> MLQFEIDDEMEPLYNQAKQMRYGDYMKSTFKEDHSLEHRCVESAKIRAKYPDRVPVIVEKVSGSQIVDIDKRKYLVPSDITVAQFMWIIRKRIQLPSEKAIFLFVDKTVPQSSLTMGQLYEKEKDEDGFLYVAYSGENTFGLEVLFQ

Mammals conserve multiple mammalian Atg8-family proteins (mATG8s) consisting of GABARAP (GABA type A receptor-associated protein) and MAP1LC3/LC3 (microtubule associated protein 1 light chain 3) subfamilies that tightly bind to autophagic membranes in a membrane-anchored form. These proteins are crucial for selective autophagy and recruit proteins bearing LC3-interacting region (LIR) motifs. Many mATG8-interacting proteins contain canonical LIR motifs that have a basic hydrophobic LIR motif with a core consensus sequence of (W/F/Y)-X-X-(L/I/V), which binds to the W- and L-sites conserved in mATG8 proteins using the amino acids W/F/Y and L/I/V, respectively. In this study, we identified LIR motifs specific to the membrane-anchored form of each mATG8 and characterized the residues critical for their selective interaction using cell-based assays and structural analyses.

An atypical LIR motif from SpHfl1 (LIR[Sp]), which binds to Atg8 in yeast, was mostly localized to GABARAPL2- and weakly but significantly localized to GABARAP- and GABARAPL1-containing autophagic membranes. Isothermal titration calorimetry (ITC) experiments further confirmed the strong and specific binding affinity of LIR(Sp) to GABARAPL2; the dissociation constant (Kd) of LIR(Sp) to GABARAPL2 was 0.24 μM, which was 8–12 times lower than that to GABARAP (1.8 μM) and GABARAPL1 (2.9 μM). We successfully determined the structure of the LIR(Sp)-GABARAPL2 fusion protein at a resolution of 1.86 Å. The structure of the LIR(Sp)-GABARAPL2 complex is similar to that of the LIR(Sp)-SpAtg8 complex. The SpHfl1 LIR consists of an α-helix, from D391 to M404, and an N-terminal tail. The helix formed extensive hydrophobic interactions with V51, P52, I55, W62, and I63 of GABARAPL2 using M394, L397, Y398, A401, and M404. Among these, Y398 formed the most critical interaction, as it was inserted deep into the L-site pocket of GABARAPL2. In addition to hydrophobic interactions, three acidic residues of LIR(Sp), D391, E393, and E395, formed electrostatic interactions with K46, R67, and R28 in GABARAPL2, respectively. Although most of the interactions were similar to those in the LIR(Sp)-SpATG8 structure, F388 of SpHfl1 was not inserted into the W-site of GABARAPL2. Among the GABARAPL2 residues involved in the interaction with LIR(Sp), W62 was the sole residue that was not conserved in other mATG8 proteins (F, K, or S was also observed at this position).>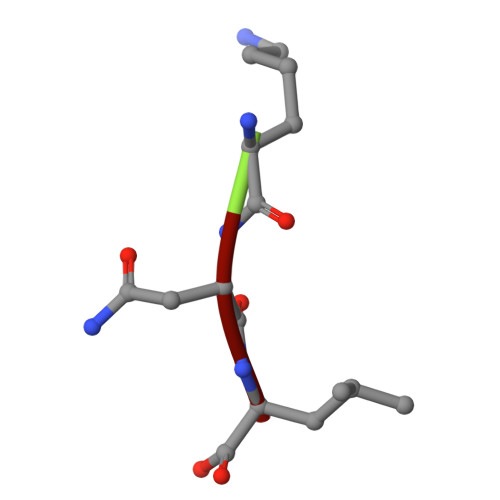 KNL>[2x]MTDAELSPTDWVREQTERILEQGTTDGVHVLDRPIVLFTTTGAKSGKKRYVPL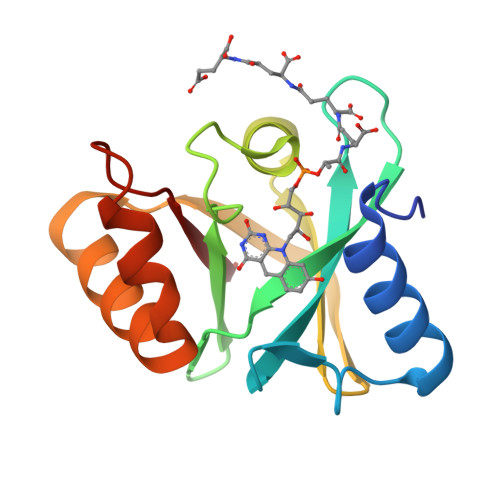MRVEENGKYAMVASKGGDPKHPSWYFNVKANPTVSVQDGDKVLPDRTARELEGEEREHWWKLAVEAYPPYAEYQTKTDRLIPVFIVE> MSFTQANCFRPSYYPARITRPNCISS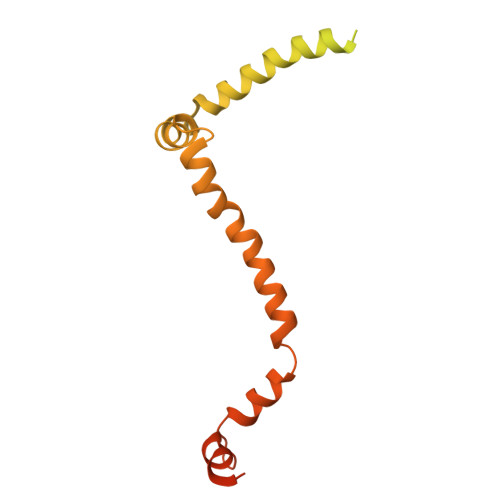VPIRSSVRFDHFPRTSFTLRATAAVSTQFSPLLDHRRRLPTGKSKQSSAVCLFGGKDKPDGSDEISPWKAIEKAMGKKSVEDMLREQIQKKDFYDTDSGGNMPPRGGGSGGGGGNGEERPEGSGGEDGGLAGIADETLQVVLATLGFIFLYTYIITGEELVKLARDYIRFLMGRPKTVRLTRAMDSWNGFLEKMSRQRVYDEYWLEKAIINTPTWYDSPEKYRRVIKAYVDSNSDEAYVESNSDEVSY> MAFKIQLDTLGQLPGLLSIYTQISLLYPVSDSSQYPTIVSTFEQGLKRFSEAVPWVAGQVKAEGISEGNTGTSFIVPFEDVPRVVVKDLRDDPSAPTIEGMRKAGYPMAMFDENIIAPRKTLPIGPGTGPDDPKPV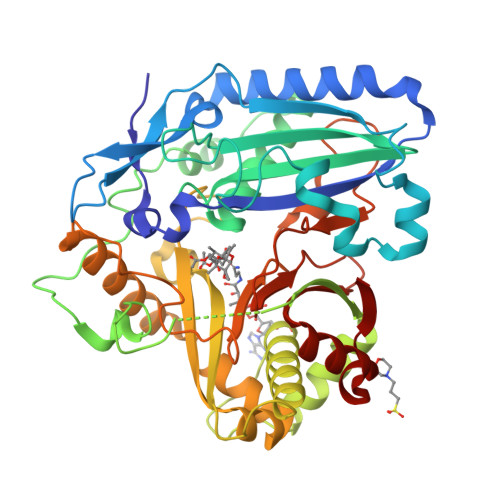ILLQLNFIKGGLILTVNGQHGAMDMVGQDAVIRLLSKACRNDPFTEEEMTAMNLDRKTIVPYLENYTIGPEVDHQIVKADVAGGDAVLTPVSASWAFFTFSPKAMSELKDAATKTLDASTKFVSTDDALSAFIWKSASRVRLERIDGSAPTEFCRAVDARPAMGVSNNYPGLLQNMTYHNSTIGEIANESLGATASRLRSELDPASMRQRTRGLATYLHNNPDKSNVSLTADADPSTSVMLSSWAKVGLWDYDFGLGLGKPETVRRPIFEPVESLMYFMPKKPDGEFCAALSLRDEDMDRLKADKEWTKYAQYVG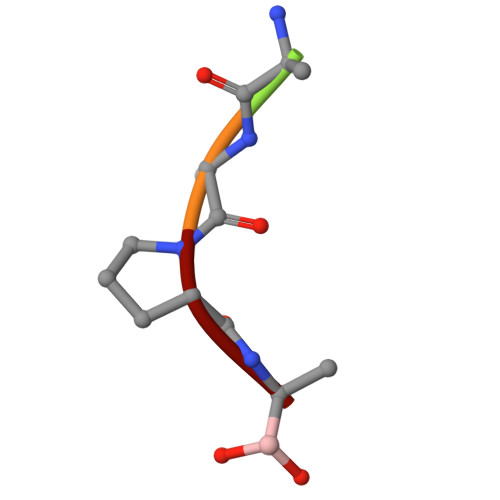> XAAPA>[2x]MAFLLALDQGTTSSRAILFTLEGRPVAVAKREFRQLYPKPGWVEHDPLEIWE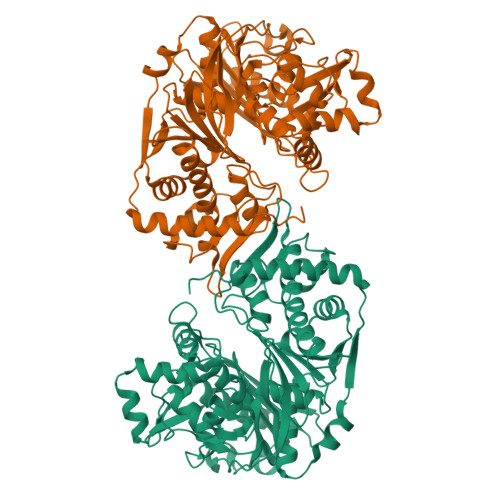TTLWAAREVLRRAGAEAGEVLALGITNQRETTLLWDRKTGKPLHNAIVWQDRRTTPLCEALRAKGLEPLFRERTGLLFDPYFSGTKLVWLLENVPGLKARAEGGGVAFGTVDTWLIWNLTGGKVHATDPTNASRTLLFNLHTLAWDPELLEALGIPAALLPEVRPSDGDFGETLPELLGAPVPIRGVLGDQQAALFGQAALGGGEGKCTYGTGAFLLLNTGKRPVLSEKGLLATVAWSLGGRATYALEGSLFVAGAAVGWLKEVGLIRESAEVEALAASVEDTGDVYFVPAFTGLGAPYWDPYARGTLLGLTRGTSRAHLARAALEGVAFQVRDVVLAMEEEAGVRLKVLKADGGMAQNRLFLKIQADLLGVPVAVPEVTETTALGAALMAGVGAGALSPEDVAGRFREAERFLPTMPEGRREALYRRWREAVERAKGWAREG>[2x]MKKIGTMLLFSILIAGCTQAQPDLKKPKKEAIATSSTQVNAPSFFHLSVLKDV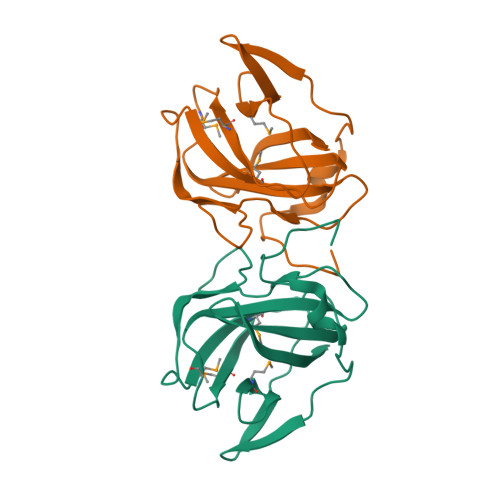NWEETPSFIQEKIPLKGIEEKIAMADSPIIANEKNEIMWYFLDPEMPTGKLSIIALKQGSVTPTPLLFQQESSEPTWTTSNTIDSTTNELPLTMSLPSSGLWVLNIYVNEKYYDQFVITAE>AMTTRNNNNVLAVSKKQLGVLAASAAVGALRNYIGESSPALLQSAVGLGKKALNKVRNRRKQGNQQIITHVGGVGGSIMAPVAVSRQLVGSKPKFTGRTSGGVTVTSHREYLTQVNNSSGFVVNGGIVGNSLQLNPSNGTLFSWLPALASNFDQYSFNSVVLDYVPLCGTTEVGRVALYFDKDSQDPEPADRVELANFGVLKETAPWAEAMLRIPTDKVKRYCNDSATVDQKLIDLGQLGIATYGGAGADAVGELFLARSVTLYFPQPTNTLLSSKRLDLTGSLADATGPGYLVLTRTPTVLTHTFRATG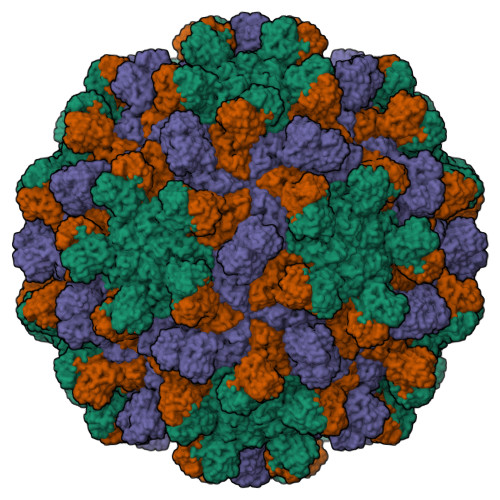TFNLSGGLRCLTSLTLGATGAVVINDILAIDNVGTASDYFLNCTVSSLPATVTFTVSGVAAGILLVGRARANVVNLL[3x]N-(4-chloro-2,5-dimethoxyphenyl)acetamide 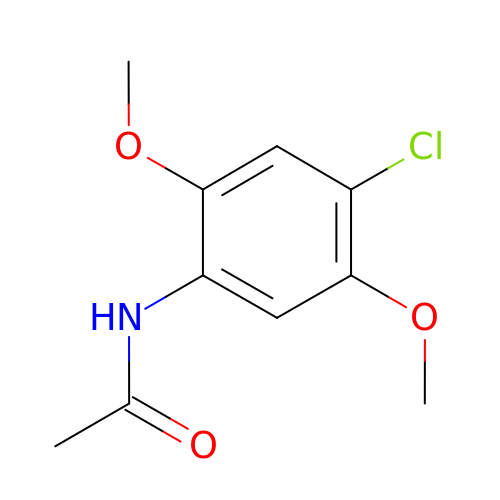| C10 H12 Cl N O3 | OQKSIDOPPLSAOL-UHFFFAOYSA-N> GPTPEAPYASLTEIEHLVQSVCKSYRETCQLRLEDLLRQRSNIFSREEVTGYQRKSMWEMWERCAHHLTEAIQYVVEFAKRLSGFMELCQNDQIVLLKAGAMEVVLVRMCRAYNADNRTVFFEGKYGGMELFRALGCSELISSIFDFSHSLSALHFSEDEIALYTALVLINAHRPGLQEKRKVEQLQYNLELAFHHHLCKTHRQSILAKLPPKGKLRSLCSQHVERLQIFQHLHPIVVQAAFPPLYKELFSTE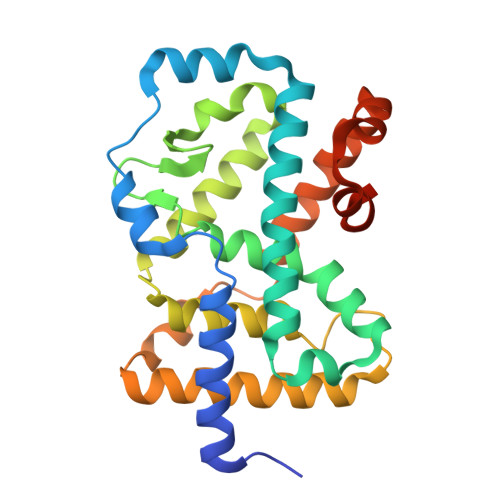TESPVGLSK> GSMVPPPENVRMNSVNFKNILQWESPAFAKGQLTFTAQYLSYRIFQDKCMQTTLTECDFSSLSKYGDHTLRVRAEFADEHSDWVQITFCPVDDTIIGPPGMQVEVLADSLHMRFLAPKIENEYETWTMKDMYNSWTYNVQYWKQG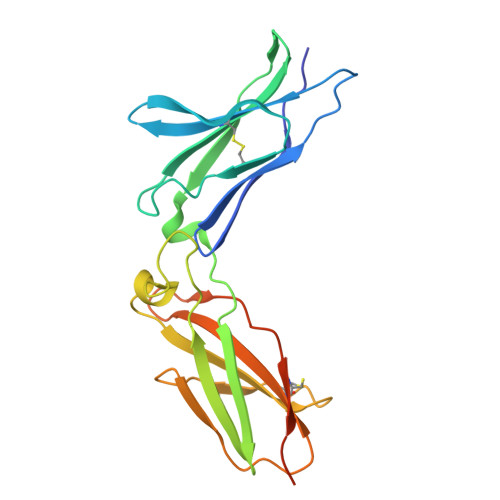TDEKFQITPQYDFEVLRNLEPRTTYCVQVRGFLPDRNKAGEWSEPVCEQTTHDETVPSAAAHHHHHH6-[2-[5-[2-(dimethylamino)ethyl]pyridin-3-yl]ethyl]-4-methyl-pyridin-2-amine 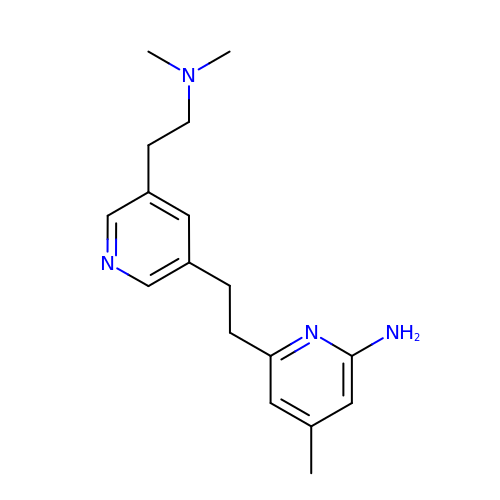| C17 H24 N4 | DKMOHXHCZRXLEY-UHFFFAOYSA-N>[5x]TTQPALLRLSDHLLANYKKGVRPVRDWRKPTTVSIDVIMYAILNVDEKNQVLTTYIWYRQYWTDEFLQWTPEDFDNVTKLSIPTDSIWVPDILINEFVDVGKSPNIPYVYVHHRGEVQNYKPLQLVTACSLDIYNFPFDVQNCSLTFTSWLHTIQDINITLWRSPEEVRSDKSIFINQGEWELLEVFPQFKEFSIDISNSYAEMKFYVIIRRRPLFYAVSLLLPSIFLMVVDIVGFCLPPDSGERVSFKITLLLGYSVFLIIVSDTLPATAIGTPLIGVYFVVCMALLVISLAETIFIVRLVHKQDLQRPVPDWLRHLVLDRIAWILCLGEQPMAHRPPATFQANKTDDCSAMGNHCSHVGGPQDLEKTPRGRGSPLPPPREASLAVRGLLQELSSIRHFLEKRDEMREVARDWLRVGYVLDRLLFRIYLLAVLAYSITLVTLWSIWHYS

Serotonin binds to serotonin receptors (5-HT3Rs), a pentameric ligand-gated ion channel (pLGIC), on the vagal afferent nerve in the gut and on the chemoreceptor trigger zone in the brainstem leading to severe nausea and vomiting in patients receiving cancer treatments. Setrons, competitive antagonists of 5-HT3R, are effective in the prevention of chemotherapy-induced nausea and vomiting (CINV), radiation therapy- induced nausea and vomiting (RINV), and postoperative nausea and vomiting (PONV). In the present study, we have solved cryo-EM structures of the full-length 5-HT3AR in complex with palonosetron, ondansetron, and alosetron at the resolution range of 2.9 Å to 3.3 Å. Overall, setrons stabilize 5-HT3AR conformational states that are non-conductive, but appear to lie between the apo and serotonin-bound states.

The isoquinoline derivative palonosetron, the only FDA approved second generation setron, is shown to have a longer half-life, improved bioavailability, and efficacy. Iterative classifications and C5 symmetry-imposed refinement produced a final three-dimensional reconstruction at a nominal resolution of 3.3 Å for 5-HT3AR-Palono (with 91,163 particles), 3.0 Å for 5-HT3AR-Ondan (67,333 particles), and 2.9 Å for 5-HT3AR-Alo (42,065 particles). The basic amine of the setron is in a bicyclic ring in granisetron and palonosetron, and a diazole ring in ondansetron and alosetron. The aromatic end of the molecule is an indazole in granisetron, isoquinoline in palonosetron, carbazole in ondansetron, and pyridoindole in alosetron. In contrast, most setron molecules maintained a low RMSD (RMSD average values of 1.1 Å, 1.0 Å, and 1.1 Å for granisetron, ondansetron, and alosetron, respectively), with palonosetron demonstrating the largest RMSD (1.9 Å) among all the simulated setrons. During the simulation, the palonosetron’s bicyclic ring displayed fluctuation and positional reorientation. In these orientations, palonosetron had distinct interactions with binding-site residues, in particular with Asn101 in the ‘down’ position and Trp156 in the ‘up’ position. In 5-HT3AR-Palono, the tertiary amine on the ligand’s bicyclic ring makes water-mediated and direct polar contacts with the backbone oxygen of Trp156 or the sidechain of Asn101 depending on the orientation of bicyclic ring. The carbonyl group of the isoquinoline moiety interacts with the amine nitrogen of Trp156 and carbonyl oxygen of Tyr64 through a water molecule. Palonosetron forms an apolar interaction with Arg169 with higher probability compared to the other ligands, potentially due to palonosetron’s pose forming weak interactions with loop C in favor of loop F. In 5-HT3AR-Ondan, the ondansetron molecule forms highly probable edge-to-face stacking interactions with Tyr126 and Tyr207.>ASHMFRKLAAECFGTFWLVFGGCGSAVLAAGFPELGIGFAGVALAFGLTVLTMAFAVGHISGGHFNPAVTIGLWAGGRFPAKEVVGYVIAQVVGGIVAAALLYLIASGKTGFDAAASGFASNGYGEHSPGGYSMLSALVVELVLSAGFLLVIHGATDKFAPAGFAPIAIGLALTLIGLISIPVTNFSVNPARSTAVAIFQGGWALEQLWFFWVVPIVGGIIGGLIYRTLLE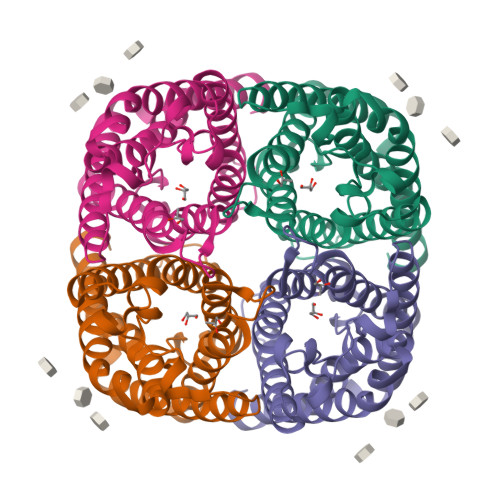KRD[2x]> MTQAWLWIGVISMALGSVFFGFGAH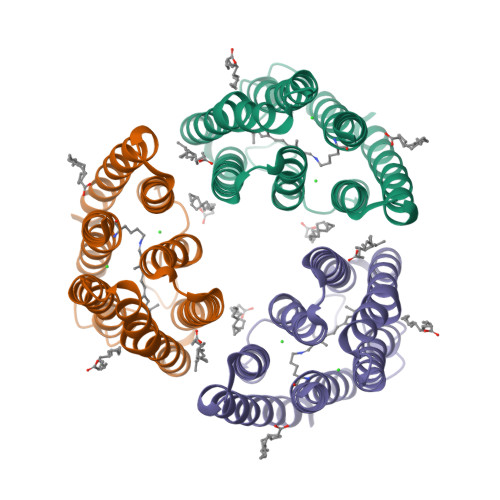NAKNERWQILYTLNFFICLIAAGLYLAMALGLGVNVIAGRPTYWVRFVTWFCSTPLLLLDLTFLGRTSLPLTGSLLGANAYMLVTGFVATVTAKPMSYIWYIVSCAAYLAIVYLLAQPYRIAAERKHPRSKQAFRTLVTVHLVLWTLYPIVWILSPEGFSTFTQGSETMFYTLLDIASKVGFGFLSLNTLHTLEQATEPARETHLSY> GSHMAIVKVTDADFDSKVESGVQLVDFWATWCG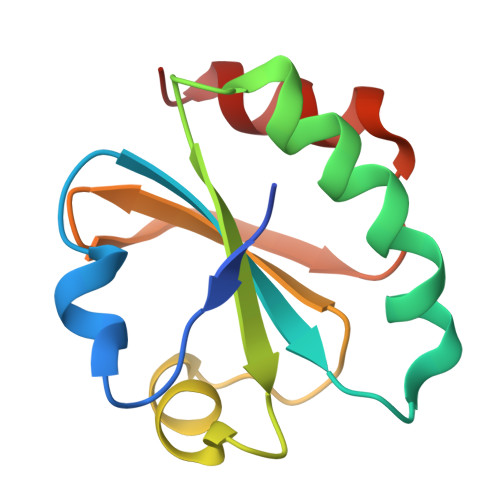TSKMIAPVLEELAADYEGKADILKLDVDENPSTAAKYEVMSIPTLIVFKDGQPVDKVVGFQPKENLAEVLDKHL6-benzyl-1-cyclopentyl-1,5-dihydro-4H-pyrazolo[3,4-d]pyrimidin-4-one 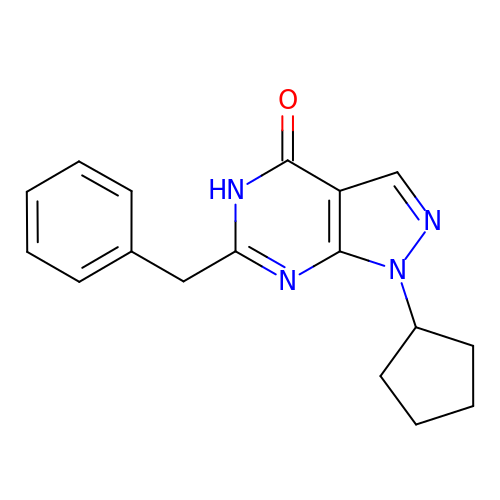| C17 H18 N4 O | FVOYQCUKGQGDKH-UHFFFAOYSA-N> MVNYCRLPCRGDNYHVGCGEPAYAQECGQSPRTRELLKEHRNEILSKINDVRDHVAKGSWGLPVAARMKVVVWDAELAGLAKRHTKGCVGETHACRNTERFWLPGQLNFKYSGDKLPRIKELIDDAVKKGHLQKHNITREIIENYRENGPNGDVKELALAISDRVTAVGCGLTTWEDGAKARALLTCNFSSQNTRGRPVYK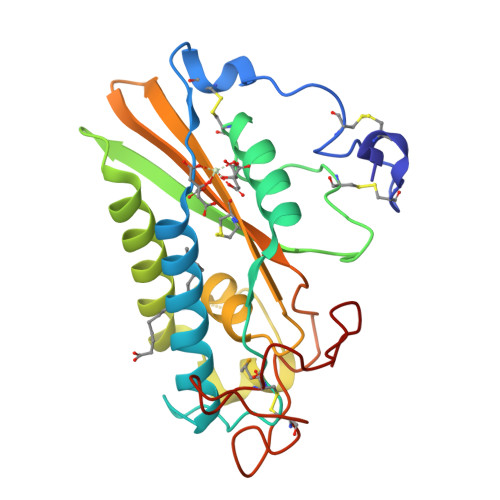IGNSPGEKCIEKDETYKNLCSATEPIDPNKSN> DRIDVLKGEKALKASGLVPEHADAFKKIARELNTYILFRPVNKLATNLIKSGVATKGLNVHGKSSDWGPVAGYIPFDQDLSKKHGQQLAVEKGNLENKKSITEHEGEIGKIPLKLDHLRIEELKENGIILKGKKEIDN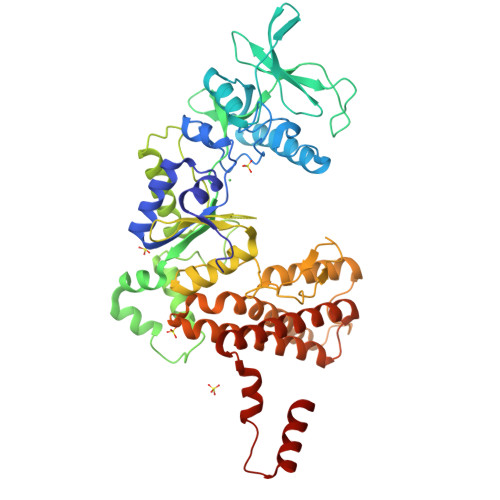GKKYYLLESNNQVYEFRISDENNEVQYKTKEGKITVLGEKFNWRNIEVMAKNVEGVLKPLTADYDLFALAPSLTEIKKQIPQKEWDKVVNTPNSLEKQKGVTNLLIKYGIERKPDSTKGTLSNWQKQMLDRLNEAVKYTGYTGGDVVNHGTEQDNEEFPEKDNEIFIINPEGEFILTKNWEMTGRFIEKNITGKDYLYYFNRSYNKIAPGNKAYIEWTDPITKAKINTIPTSAEFIKNLSSIRRSSNVGVYKDSGDKDEFAKKESVKKIAGYLSDYYNSANHIFSQEKKRKISIFRGIQAYNEIENVLKSKQIAPEYKNYFQYLKERITNQVQLLLTHQKSNIEFKLLYKQLNFTENETDNFEVFQKIIDEK>MDYTVGTYLAERLVQIGLKHHFAVAGDYNLVLLDNLLDNKNMEQVYCCNELNCGFSAEGYARAKGAAAAVVTYSVGALSAFDAIGGAYAENLPVILISGAPNNNDHAAAHVLHHALGKTDYHYQLEMAKNITAAAEAIYTPEEAPAKIDHVIKTALREKKPVYLEIACNIASMPCAAPGPASALFNDEASDEASLNAAVEETLKFIENRDKVAVLVGSKLRAAAAEEAAVKFADALGGAVATMAAAKSFFPEENPHYIGTSWGEVSYPGVEKTMKEADAVIALAPVFNDYSTTGWTDIPDPKKLVLAEPRSVVVNGIRFPSVHLKDYLTRLAEKVSKKTGALDFFKSLNAGELKKADPADPSAPLVNAEIARQIEDLLTPNTTVIAETGDSWFNAQRMKLPNGARVEYEMQWGHIGWSVPAAFGYAVGAPERRNILMVGDGSFQLTAQEVAQMVRLKLPVIIFLINNYGYTIEVMIHDGPYNNIKNWDYAALMEVFNGNGGYDSGAGKGLKAKTAAELEEAIKVALDNTDGPTLIECFIAREDCTEELVKWGERVAAANSRKPVNKLLLEHHHHHH[2x]

Pyruvate decarboxylase (PDC) converts pyruvate to acetaldehyde through nonoxidative decarboxylation, a reaction that typically occurs in anaerobic fermentations. PDC self-associates to form a 260 kDa dimer of dimers, with two active sites buried at each dimer interface. In addition, the monomeric unit of PDC is composed of three distinct structural regions. In this study, we used iterative computational protein design to rationally engineer the mesophilic enzyme, pyruvate decarboxylase, to exhibit enhanced thermal endurance at the growth temperature of a thermophilic organism.

A significant increase in thermal stability is observed with PDC2.03, which combines PDC1.01, PDC1.10 and the additional four substitutions. PDC2.03 contains sixteen mutations in the monomeric unit and sixty-four mutations in the homotetrameric complex. The mutations are found throughout the PDC complex as well as in each of the three structural regions of the monomeric unit. The structure of PDC2.03 was refined to a resolution of 1.67 Å with R and Rfree of 0.170 and 0.203, respectively. There are two molecules in the asymmetric unit in complex with TPP and magnesium. Each monomer has three domains with an open α/β topology with several ethylene glycol and sulfate molecules on the surface. The backbone root-mean-square deviation (RMSD) between chain A of the wild-type PDB and PDC2.03 is 0.19 Å. The largest conformational difference, located in the upper left of Fig. 5c, is located at a crystal contact point and distant from both the active sites and any of the 16 mutations. Thus, the mutations impart significant enhancement in thermal stability without unintended structural alterations. PDC2.03, which displayed no loss of molar ellipticity until 90 °C when monitored by CD, lasted 60 min at 60 °C before entering phase 2, and never entered phase 3 for the duration of the experiment.> GSDAPDEFRDPLMDTLMTDPVRLPSGTIMDRSIILRHLLNSPTDPFNRQTLT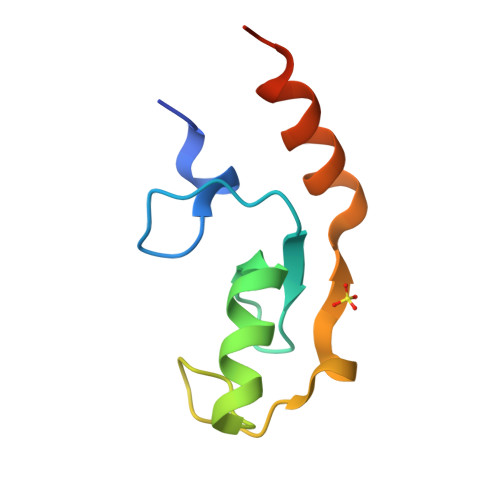ESMLEPVPELKEQIQAWMREKQNSDH> RRGLLPNHIWQGDVTHYKYKKYK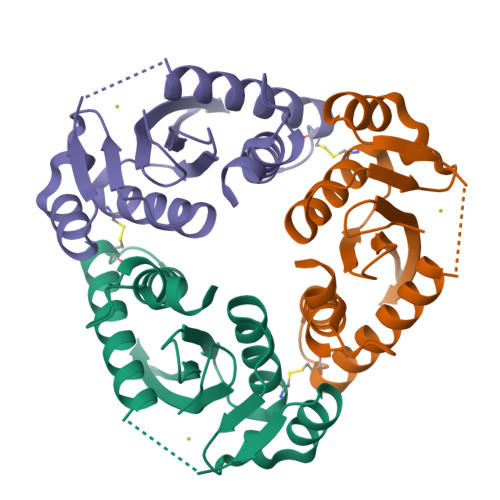YCLHVWVDTFSGAVSVSCKKKETSCETISAFLQAISLLGKPLHINTDNGPAFLSQEFQEFCTSYHIKHSTHIPYNPTSSGLVERTNGIIKNLLNKYLLDCPNLPLDNAINKALWTLNQLNVMNPSGKTRWQIHHSPPLPPIPEAST> MAHHHHHHVDDDDKENLYFQSKPNLSAKDLALLLFTHLPGNNTPFHILAQVLSKIAYKSGKSGAFLDAFHQILSEGENAQAALTRLSRTFDAFLGVVPPVIRVKNF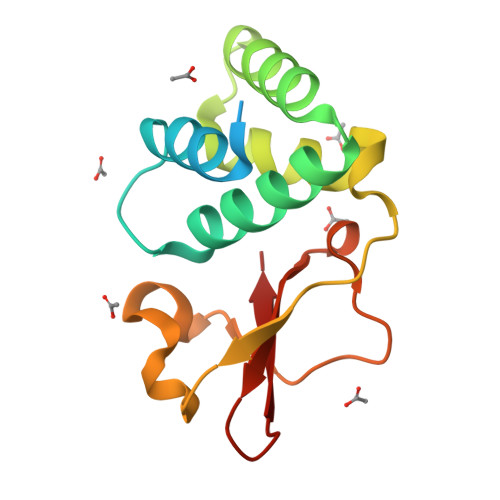QTVPRPCQKSLRAVPPNPTIDKGWVCVYSSEQGETRALKI> MNPFQKNESKETLFSPVSIEEVPPRPPSPPKKPSPTICGSNYPLSIAFIVVNEFCERFSYYGMKAVLILYFLYFLHWNEDTSTSIYHAFSSLCYFTPILGAAIADSWLGKFKTIIYLSLVYVLGHVIKSLGALPILGGQVVHTVLSLIGLSLIALGTGGIKPCVAAFGGDQFEEKHAEERTRYFSVFYLSINAGSLISTFITPMLRGDVQCFGEDCYALAFGVPGLLMVIALVVFAMGSKIYNKPPPEGNIVAQVFKCIWFAISNRFKNRSGDIPKRQHWLDWAAEKYPKQLIMDVKALTRVLFLYIPLPMFWALLDQQGSRWTLQAIRMNRNLGFFVLQPDQMQVLNPLLVLIFIPLFDFVIYRLVSKCGINFSSLRKMAVGMILACLAFAVAAAVEIKINEMAPAQPGPQEVFLQVLNLADDEVKVTVVGNENNSLLIESIKSFQKTPHYSKLHLKTKSQDFHFHLKYHNLSLYTEHSVQEKNWYSLVIREDGNSISSMMVKDTESRTTNGMTTVRFVNTLHKDVNISLSTDTSLNVGEDYGVSAYRTVQRGEYPAVHCRTEDKNFSLNLGLLDFGAAYLFVITNN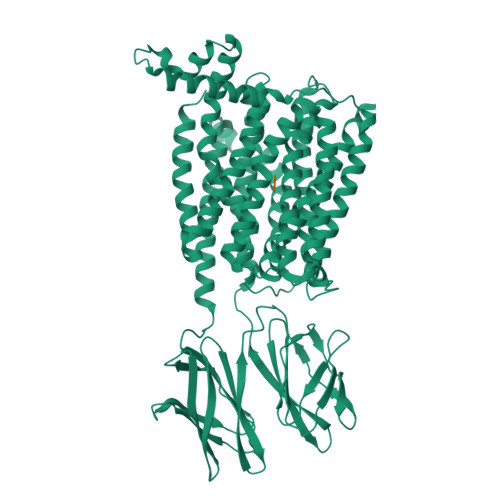TNQGLQAWKIEDIPANKMSIAWQLPQYALVTAGEVMFSVTGLEFSYSQAPSSMKSVLQAAWLLTIAVGNIIVLVVAQFSGLVQWAEFILFSCLLLVICLIFSIMGYYYVPVKTEDMRGPADKHIPHIQGNMIKLETKKTKL;> AF>[4x]ALTEKDLKNLPEDGIDSENPGKYRNLLNDLQGNILKGHGRDHSVHLFLQFKPEQVEVVKQWIQSFAQTYITSAKKQADEAFKYRQKGVSGDVFANFFLSRHGYEYLEIEPFQIPGDKPFRMGMKNEEIRSSLGDPKIATWELGFQSEIHALVLIADDDIVDLLQIVNQITQKLRQIAEIVHREDGFILRNQAGQIIEHFGFVHGVSQPLF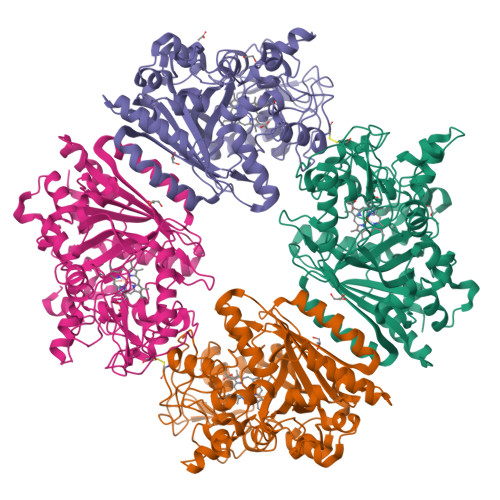MKRDVVRERVNNCDFDKWDPKAPLDSILVEDPNGNTKDSYGSYLVYRKLEQNVKAFREDQRKLAQKLNIQENLAGALIVGRFADGTPVTLSDIPTYAVTPTNNFNYDGDLAATKCPFHSHTRKTNPRGDTARLLTTDGHFDEAFKEERGHRITRRAVSYGENNPSKEPVSGSGLLFLCFQSNIENQFNFMQSRWANPQNFVQVNTGPDPLIGQPSGTQKWPKKWGEPETEEYNFQLWINMKGGEYFFAPSISFLKTLA Triosephosphate isomerase (TPI or TIM) is a functionally and structurally well-known enzyme that plays a crucial role in glycolytic and gluconeogenic metabolism. TPI accurately and efficiently interconverts dihydroxyacetone phosphate (DHAP) and glyceraldehyde-3-phosphate (GAP). The overall structure of TaTPI protomer confirms to the canonical TIM-barrel fold with eight α-helices and eight parallel β-strands from 216 amino acid residues. Unlike other thermostable archaeal TPIs, TaTPI forms a stable dimer in solution, which we confirmed using analytical ultracentrifugation and size-exclusion chromatography.

In this work, we report crystal structures of apo- and glycerol-3-phosphate (G3P)-bound TaTPI, each representing open and closed form. The crystal structures of apo-TaTPI and its complex with glycerol-3-phosphate (G3P), an analogue of the substrate glyceraldehyde-3-phosphate, have been determined at 1.94 and 2.17 Å resolution, respectively. Crystal structures of apo- and G3P-bound TaTPI contain four copies of TaTPI monomer in the asymmetric unit, comprising two homodimers. Overall structures of apo- and G3P-bound TaTPI were similar with r.m.s.d. of 0.69 Å for 216 Cα positions, except G3P-bound area. In addition, water molecules around the active site of apo-TaTPI are expelled from the active site and would be replaced with substrate upon substrate binding. In the crystal structure of apo-TaTPI, Cys50 in helix 2 of each homodimer drew our attention since it interacts with the other Cys50 from adjacent TaTPI homodimer via sulfur-containing hydrogen bonds, not disulfide bonds. Thus, we needed to re-confirm the oligomeric status of apo-TaTPI to make it sure whether the interaction of Cys-Cys is physiologically relevant or crystallographic artefact. To verify the oligomeric state of apo-TaTPI in solution, analytic ultracentrifugation analysis (AUC) was performed. Data analysis using the reversible model (Eq 2) gave large negative Ink values for monomer-dimer (1x-2x) and monomer-trimer (1x-3x) models and much higher RMS values (~10−2), so the reversible models for monomer-dimer (1x-2x) and monomer-trimer (1x-3x) equilibrium would not be the case for TaTPI. These results strongly indicate that apo-TaTPI exits as homogeneous dimer in solution. In addition, analytical size-exclusion chromatography results of apo-TaTPI, which were confirmed at two different TaTPI protein concentrations (0.9 and 4.5 mg ml-1), also supported the dimeric conformation in solution.

>[4x]MDMYTAIVNLKTYREATGANFTRFMEKFEPVQGKFELIFSPSLLDLEKAAKCGKFRFFAQHVDAEPYGAYTGHVPMDMMIDLGITGSILNHSERRLPRDTIINTLKKASKLDFTIVLCVENAEEAKYFREYEPDFIAYEPRDLIGGDVSVSTAKPEIIEDIVKIYEGTGTSVLVGAGIKTGEDVRRSIGLGARGILVASGVVKSADPTKSLNSLIELKLEHHHHHH Expanding this pattern to hpphhph can produce larger α-helical barrels. Here, we show that pentameric to nonameric barrels are accessed by varying the residue at one of the h sites. In peptides with four L/I–K–E–I–A–x–Z repeats, decreasing the size of Z from threonine to serine to alanine to glycine gives progressively larger oligomers. X-ray crystal structures of the resulting α-helical barrels rationalize this: side chains at Z point directly into the helical interfaces, and smaller residues allow closer helix contacts and larger assemblies.

Our hypothesis was that these should direct larger and smaller oligomers, respectively. Encouragingly, the new Thr@g sequences consistently scored best as pentamers: for the a = d = Ile variant the pentameric assembly was favoured outright; while the a = Leu, d = Ile variant scored equally well as pentamer or hexamer. We determined X-ray protein crystal structures for all Gly@g and Thr@g variants. As predicted, the Thr@g peptides formed parallel pentamers (Fig. 3 and Tables S4 and S5†). Summarizing these data, Type-2 CC peptides with sequence repeats LppIApZ and Z = Thr, Ser, or Ala, form pentameric, hexameric, and heptameric αHBs, respectively. The average distance increases from 8.0 ± 0.1 Å in the Gly@g nonamer to 10.4 ± 0.1 Å in the Thr@g pentamer.

>XGEIAQTLKEIAKTLKEIAYTLKEIAQTLKGX[5x]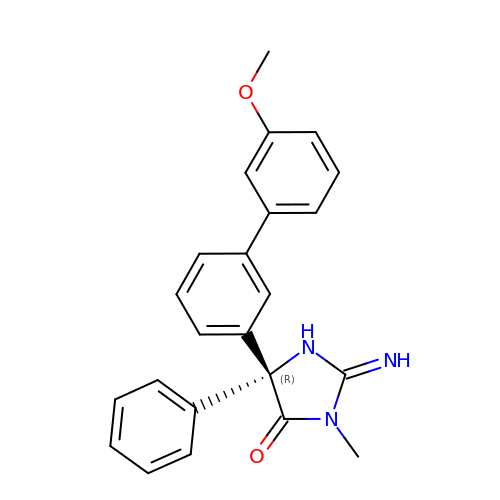(2E,5R)-2-imino-5-(3'-methoxybiphenyl-3-yl)-3-methyl-5-phenylimidazolidin-4-one | C23 H21 N3 O2 | LRYKHTDVFXMHEH-HSZRJFAPSA-N> MQNITQSWFVQGMIKATTDAWLKGWDERNGGNLTLRLDDADIAPYHDNFHQQPRYIPLSQPMPLLANTPFIVTGSGKFFRNVQLDPAANLGIVKVDSDGAGYHILWGLTNEAVPTSELPAHFLSHCERIKATNGKDRVIMHCHATNLIALTYVLENDTAVFTRQLWEGSTECLVVFPDGVGILPWMVPGTDAIGQATAQEMQKHSLVLWPFHGVFGSGPTLDETFGLIDTAEKSAQVLVKVYSMGGMGQTISAAELIALGKR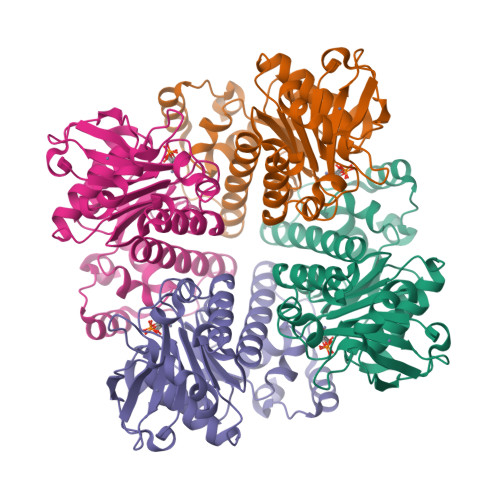FGVTPLASALAL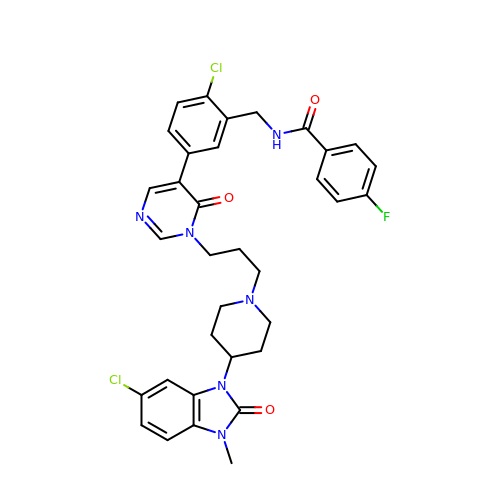N-[2-chloro-5-(1-{3-[4-(6-chloro-3-methyl-2-oxo-2,3-dihydro-1H-benzimidazol-1-yl)piperidin-1-yl]propyl}-6-oxo-1,6-dihydropyrimidin-5-yl)benzyl]-4-fluorobenzamide | C34 H33 Cl2 F N6 O3 | UUSUCXDJVSXCBL-UHFFFAOYSA-N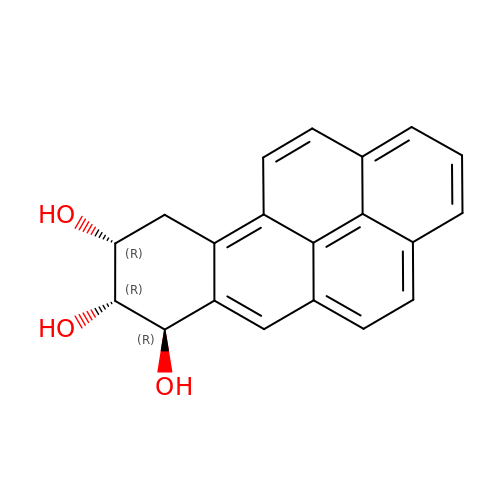1,2,3-TRIHYDROXY-1,2,3,4-TETRAHYDROBENZO[A]PYRENE | C20 H16 O3 | GFANZDFKCCJYRF-NSISKUIASA-N>[4x]MSVGIVYGDQYRQLCCSSPKFGDRYALVMDLINAYKLIPELSRVPPLQWDSPSRMYEAVTAFHSTEYVDALKKLQMLHCEEKELTADDELLMDSFSLNYDCPGFPSVFDYSLAAVQGSLAAASALICRHCEVVINWGGGWHHAKRSEASGFCYLNDIVLAIHRLVSSTPPETSPNRQTRVLYVDLDLHHGDGVEEAFWYSPRVVTFSVHHASPGFFPGTGTWNMVDNDKLPIFLNGAGRGRFSAFNLPLEEGINDLDWSNAIGPILDSLNIVIQPSYVVVQCGADCLATDPHRIFRLTNFYPNLNLDSDCDSECSLSGYLYAIKKILSWKVPTLILGGGGYNFPDTARLWTRVTALTIEEVKGKKMTISPEIPEHSYFSRYGPDFELDIDYFPHESHNKTLDSIQKHHRRILEQLRNYADLNKLIYDYDQVYQLYNLTGMGSLVPR

In our study, we show that Schistosoma mansoni histone deacetylase 8 (smHDAC8) is a functional acetyl-L-lysine deacetylase that plays an important role in parasite infectivity and is therefore a relevant target for drug discovery. The smHDAC8 adopts a fold similar to hHDAC8 (r.m.s.d. on Cα's of 1.2 Å between the human and schistosome enzymes), forming a single α/β domain composed of a central, eight-stranded parallel β-sheet sandwiched by 15 α-helices (α1–α15). In smHDAC8 these three ions and their coordinating residues are conserved, thus reinforcing the similarity between the human and schistosome HDAC8 enzymes. Therefore, the flipped-out conformation of smHDAC8 F151 appears to be highly specific to the schistosome enzyme in contrast to human HDACs, suggesting that this feature, together with the specific replacement of human M274 by schistosome H292, could provide the basis for the design of specific inhibitors targeting smHDAC8.

Crystals were obtained that belonged to space group P1 and which diffracted to 1.8 Å resolution. The final model contains four independent non-crystallographic monomers (r.m.s.d. on Cα's from 0.1 to 0.6 Å), and has good deviations from ideal geometry, with R-factor and R-free values of 0.15 and 0.19. We were able to crystallize smHDAC8 in a non-inhibited form. However, we observed in our electronic density the unambiguous presence of an L-tartrate molecule provided by the crystallization buffer which was bound in the smHDAC8 active site where it coordinated the catalytic zinc ion. Our structural data suggest that HDAC8 enzymes display some flexibility at their active sites, which could explain that small molecules (e.g. L-tartrate in our native form and inhibitors in the other cases) coordinating the catalytic zinc are required to stabilize the protein and support crystallization. First, as expected, we observe the replacement of M274 by H292 in smHDAC8 that diminishes the hydrophobic character of the pocket that normally accommodates the aliphatic part of the incoming acetylated lysine. Further, while the position of smHDAC8 D100 is similar to that of its human counterpart, D101, we observe a change in conformation of the smHDAC8 Y341 side chain compared to hHDAC8 Y306. In contrast, the smHDAC8 Y341 side chain points towards the rim of the catalytic pocket. The most striking and certainly least expected difference concerns the smHDAC8 F151 side chain that is turned away from the catalytic pocket and is inserted into a smaller hydrophobic pocket formed by loops that surround the active site. In the schistosome HDAC8 enzymes, this leucine is replaced by a serine (S18). This smaller residue enlarges the pocket accommodating the F151 side chain, enabling it to adopt its observed flipped-out conformation.>YKKAGLQRTLVLIKPDAFERSLVAEIMGRIEKKNFKIVSMKFWSKAPRNLIEQHYKEHSEQSYFNDNCDFMVSGPIISIVYEGTDAISKIRRLQGNILTPGTIRGDLANDIRENLIHASDSEDSAVDEISIWFPET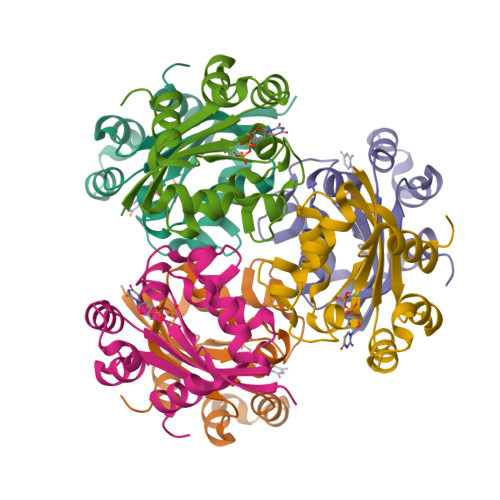KMETDN[6x]The Opp ABC transporter comprises the periplasmic binding protein (OppA), two transmembrane domains (TMDs) that span the inner membrane (OppB and OppC) and two cytosolic nucleotide-binding domains (NBDs) that drive ATP hydrolysis (OppD and OppF). Peptide-bound OppA docks to the TMDs, triggering ATP-binding and substrate translocation into the cytosol. OppA is known to promiscuously bind 2- to 5-amino-acid-long peptides, favouring positively charged side chains. We demonstrate that isopeptide-linked tripeptides (Z-XisoK, where Z and X are natural or non-canonical residues) are actively imported into E. coli via the oligopeptide permease (Opp) and processed intracellularly, resulting in high accumulation of Z and XisoK.

The structure shows a good overlap with previous ligand-bound OppA conformations and adopts the closed state, with G-SisoK enclosed in the binding pocket. G-SisoK engages in extensive interactions with OppA through its backbone and termini. The N-terminal glycine forms key hydrogen bonds and electrostatic contacts: its protonated α-amine interacts with D445, whereas the C-terminal carboxylate is stabilized by hydrogen bonds involving the side chains of R439, H397 and N392. Expression of wild-type OppA fully restored sfGFP expression with G-SisoK, whereas the D445A variant, which disrupts the interaction with the N-terminal α-amine of G-SisoK, did not rescue expression. Mutations targeting the hydrogen-bonding network at the C terminus of G-SisoK (for example, R439A), had less pronounced effects, suggesting that the OppA binding site possesses some structural flexibility. The OppA–G-SisoK crystal structure revealed no specific interactions with the serine side chain, which is accommodated in a spacious pocket. This suggests that OppA binding and uptake rely primarily on recognition of the tripeptide backbone and termini rather than side-chain identity. Crystallographic analysis of the OppA–G-SisoK complex revealed a spacious cavity extending from the serine side chain to the N-terminal glycine. One notable exception is R439, which lies within hydrogen-bonding distance of the C terminus of the ligand and is replaced by glutamine in OppA-iso. Since the R439A mutant still supports efficient G-SisoK uptake, binding is likely to be maintained through compensatory interactions with H397 and N392, which are well positioned to interact with the lysine carboxylate of G-SisoK.

>[4x]ADVPAGVTLAEKQTLVRNNGSEVQSLDPHKIEGVPESNISRDLFEGLLVSDLDGHPAPGVAESWDNKDAKVWTFHLRKDAKWSDGTPVTAQDFVYSWQRSVDPNTASPYASYLQYGHIAGIDEILEGKKPITDLGVKAIDDHTLEVTLSEPVPYFYKLLVHPSTSPVPKAAIEKFGEKWTQPGNIVTNGAYTLKDWVVNERIVLERSPTYWNNAKTVINQVTYLPIASEVTDVNRYRSGEIDMTNNSMPIELFQKLKKEIPDEVHVDPYLCTYYYEINNQKPPFNDVRVRTALKLGMDRDIIVNKVKAQGNMPAYGYTPPYTDGAKLTQPEWFGWSQEKRNEEAKKLLAEAGYTADKPLTINLLYNTSDLHKKLAIAASSLWKKNIGVNVKLVNQEWKTFLDTRHQGTFDVARAGWCADYNEPTSFLNTMLSNSSMNTAHYKSPAFDSIMAETLKVTDEAQRTALYTKAEQQLDKDSAIVPVYYYVNARLVKPWVGGYTGKDPLDNTYTRNMYIVKHHHHHH>ADKLPYKVADIGLAAWGRKALDIAENEMPGLMRMREMYSASKPLKGARIAGCLHMTVETAVLIETLVALGAEVRWSSCNIFSTQDHAAAAIAKAGIPVFAWKGETDEEYLWCIEQTLHFKDGPLNMILDDGGDLTNLIHTKHPQLLSGIRGISEETTTGVHNLYKMMANGILKVPAINVNDSVTKSKFDNLYGCRESLIDGIKRATDVMIAGKVAVVAGYGDVGKGCAQALRGFGARVIITEIDPINALQAAMEGYEVTTMDEACKEGNIFVTTTGCVDIILGRHFEQMKDDAIVCNIGHFDVEIDVKWLNENAVEKVNIKPQVDRYLLKNGHRIILLAEGRLVNLGCAMGHPSFVMSNSFTNQVM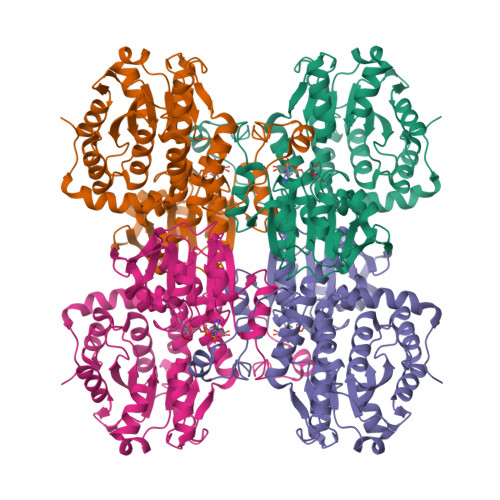AQIELWTHPDKYPVGVHFLPKKLDEAVAEAHLGKLNVKLTKLTEKQAQYLGMPINGPFKPDHYRY[4x]>[2x]GKQHVKTKSDWVIQRTPVD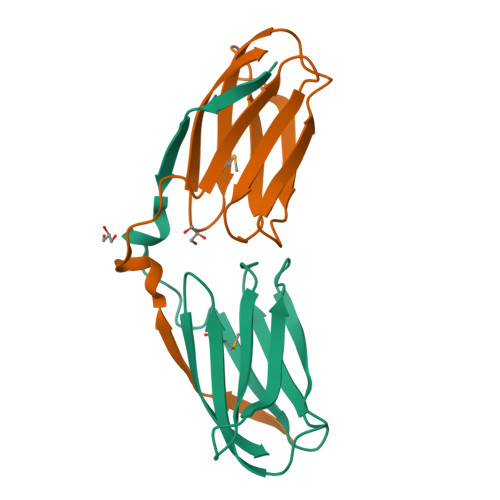PEWLKVYVDDESKRLCLNFKDSFAPITVEVKDIEKQIVFQSIIFPVAAGEYTLYLGDLSLGQYELYMYNASVKVVGNFTL>[2x]MTHTPSFDLSDIKSTLSTNVLHADDAYALENDVAPPIHISTTYTYPGTPDTLQPFTKLAEE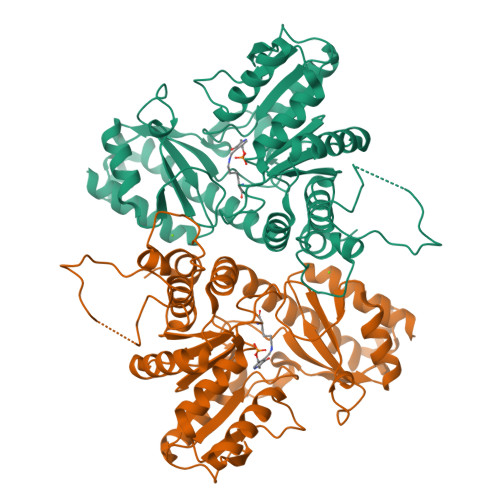DFPYYARISGNNVDRAEASLSSVLGAPSVVYSSGLAAIYGLLSYLNPKHIAVHKPGFGGYSGTIQIIARINRLTGLETSFIDGKCDAIGEGDVIWLETPLNPLGIAFDIPFYKELAKKKGAILVVDSTFAPPPIQDALVLGADYVVHSATKYLAGHSDVLAGVTASKDRSKILDLKADRAYLGTILHPQQAFLLLRSLRTFPLRIAKHSENGFLVAQHLNKLATDEQFATSLGIDSSLILEVYHNSLQTKEFVAKNLTGGHASCFSVLLKSDTVAKHLCCELKYFHHATSLGSVESLIEWRRMTDSKIDPRLVRLSIGIEDAADLIADLNRVFASLS> MGSSHHHHHHSGLVPRGSHMTSKDHVKSQIPRLSAINDLHKIWPTVEEHGAAIIESFLSLDIVRRLNEEVDPFVKIEPIPAAKTKDHPNHVLSTTTRLVNVLAPISKAYREDVLNSKVLHRICSDAFHVYGDYWVLMGAVMELAPSNPAQPLHRDMRFSHPIVEYLKPDAPATSINFLVALSPFTAENGATHVILGSHKWQNLSNV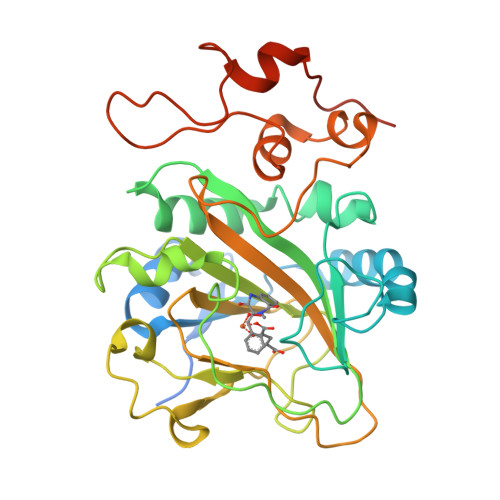SMDATVRALMNPGDALLITDSTIHCGGAETTGTETRRLLTITMGISQLTPLESNLAVPRPVIESLTPLAQRLLGWASQRSAAPRDIGLLTIRGNSIEKTMNLKAEQPLHDDEAEPLCRETI>SVLPETPVPFKSGTGAIDNDTVYIGLGSAGTAWYKLDTQAKDKKWTALAAFPGGPRDQATSAFIDGNLYVFGGIGKNSEGLTQVFNDVHKYNPKTNSWVKLMSHAPMGMAGHVTFVHNGKAYVTGGVNQNIFNGYFEDLNEAGKDSTAIDKINAHYFDKKAEDYFFNKFLLSFDPSTQQWSYAGESPWYGTAGAAVVNKGDKTWLINGEAKPGLRTDAVFELDFTGNNLKWNKLAPVSSPDGVAGGFAGISNDSLIFAGGAGFKGSRENYQNGKNYAHEGLKKSYSTDIHLWHNGKWDKSGELSQGRAYGVSLPWNNSLLIIGGETAGGKAVTDSVLITVKDNKVTVQNLEHHHHHH[2x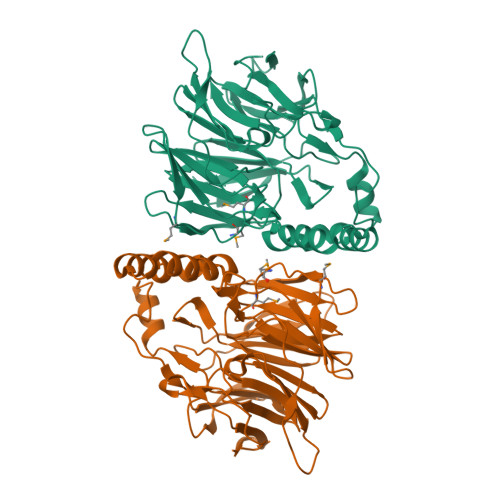]>VTQ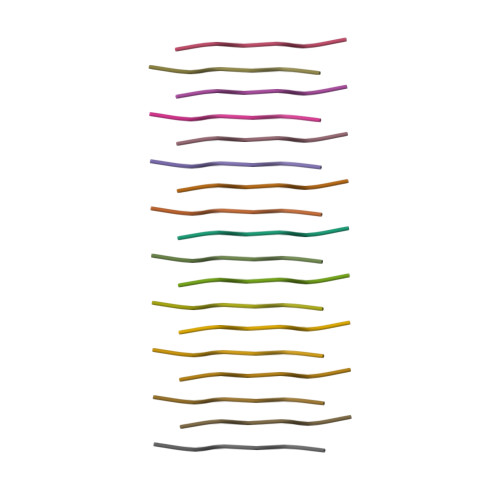VGF[2x]The molecular mechanism underlying this microtubule array reorientation involves katanin, a microtubule severing enzyme, and a plant-specific microtubule associated protein called SPIRAL2. Upon severing, SPIRAL2 binds nascent microtubule minus ends and limits their dynamics, thereby stabilizing the longitudinal array while the lateral array undergoes net depolymerization. The domain architecture of SPR2 family members is distinct from CAMSAP proteins, as the former contains a predicted N-terminal TOG domain, a central coiled-coil, and a helical C-terminal domain of unknown structure. To gain insight into SPIRAL2 structure and function, we determined a 1.8 Å resolution crystal structure of the Arabidopsis thaliana SPIRAL2 C-terminal domain.

The crystal belonged to the space group P212121, with one SPR2 molecule in the asymmetric unit, and a solvent content of 35% (calculated using the complete SPR2 649–864 construct, thus representing a lower limit for the solvent content if the construct was degraded). Selenium sites were identified and used to phase the structure, yielding clear, interpretable electron density (Final 2mFo-DFc electron density shown in Fig 3B), for which residues 717–849 (which includes the construct’s carboxy-terminal residue) were modeled. SPR2 residues 717–849 form a right-handed α-solenoid helix-turn-helix structure, composed of seven conserved α-helices (α1-α7). Six of the seven α-helices form anti-parallel helix-turn-helix pairs (α2-α3, α4-α5, and α6-α7) that pack against one another. Of these repeats, the SPR2 C-terminal domain helix-turn-helix motifs are structurally most similar to FANC repeats, as the helices are relatively straight, and lack a canonical kink present in the first helix (helix A) of a HEAT repeat, or the additional N-terminal helix (helix H1) of an ARM repeat. Collectively, conservation mapping suggests that the domain face formed by α1, α3, α5, and the α6-α7 loop is likely to constitute a functional surface, potentially for protein-protein interactions, mediated by both hydrophobic and electrostatic interactions. On the conserved face of the domain, charge is partitioned, with a basic patch localized to the α1-α3 region. The domain fold is similar to, yet structurally distinct from the C-terminal domain of Ge-1 (an mRNA decapping complex factor involved in P-body localization) and, surprisingly, the C-terminal domain of the katanin p80 regulatory subunit. Based on these differences, we do not anticipate that SPR2 engages katanin p60 using a p80-binding mode.

> GSHMGRRGWDNKASGTIRFGEGPSARSVWQASKDEATLEAIRVAGEDGAVPRPTRVAVAPEAEAMGDDDNEGQERDPIWVSWSNAMHSLRVGDIDAAYAEVLCAGDQHLVIKLMDKTGPSLDQMSNEIANEALNFISQFLLDHSLYDICLSWSQQLLELVLQDGADTFGVPMELKTEILYNLQDACSTMDPPEDWEGPAPEQLVVQLASVWEIDLQQFDK Halohydrin dehalogenases (HHDHs; also, haloalcohol dehalogenases or epoxidases, halohydrin hydrogen-halide-lyases) are biotechnologically relevant enzymes for the production of chiral epoxides and β-substituted alcohols. In their natural function, they catalyze the reversible dehalogenation of vicinal haloalcohols with formation of the corresponding epoxides. HHDHs possess a catalytic triad composed of serine, tyrosine and arginine. Protein engineering of halohydrin dehalogenase HheG for thermostabilization revealed several residues with positive impact on the apparent melting temperature.

Interestingly, whereas T123W yielded wild type-like crystals only, we obtained six different crystal forms for the T123G variant, which may already indicate an impact on the dynamic behavior of the protein. After solving and inspecting all of these crystal forms, two (T123G_1 and T123G_2) were chosen for final refinement and analysis, since they encompassed all structural changes with respect to the structure of the wild-type protein. Superimposition revealed that mutations T123G and T123W have no effect on the overall fold of the protein or on the position and orientation of the catalytic residues S152, Y165 and R169. A more thorough analysis of the variants shows that mutation of T123 to glycine or tryptophan leaves backbone hydrogen bonds to G102 and K119 unaltered, whereas side chain-specific contacts to L103, K119 and N124 are abolished. In variant T123G, on the other hand, the additional space generated by the missing side chain is partially occupied by L103, resulting in a slight displacement of a loop connecting strand β4 and helix α4 (residues 101 to 107) that covers the catalytic triad. This intricate movement could impact on substrate positioning in the active site and may hence explain the increased catalytic activity of T123G. On the other hand, the T123G variant shows the closed active site conformation already in the average structure obtained from MD simulation. At the same time, its loop mobility is significantly lower compared to variant T123W. Variant T123G was the most active one with a 5-fold higher initial reaction velocity in the azidolysis of cyclohexene oxide compared to wild-type HheG.

>[4x]AENRPVALITMATGYVGPALARTMADRGFDLVLHGTAGDGTMVGVEESFDSQIADLAKRGADVLTISDVDLTTRTGNQSMIERVLERFGRLDSACLVTGLIVTGKFLDMTDDQWAKVKAGNLDMVFHGLQAVLPPMVAAGAGQCVVFTSATGGRPDPMVSIYGGTRAGANGIVRAVGLEHARHGVQVNAIGTNYMDFPGFLKASRADGDPERRAMIEAQVPLRRLGTMDELSSVTAGLLDGSNRFQTGQFFDFSGGWGA> MAAQLSEQLAELEKRSGGRLGVAVLDTATGRRIAYRGDERFPMCSTFKALLAAAVLARVDQGKERLDRRITYGKEDLVDYSPVTEKHVGDGMTVAELCEAAITLSDNTAANLLLEALGGPAALTAFLRSIGDEVTRLDRWEPELNEAAPGDPRDTTTPAAMAATLRTLLLGDALSPASRQQLVDWLVANKTGDKRLRAGLPADWRVGDKTGTGGHGTTNDIAVIWPPGRAPIVVTVYLTESQVDA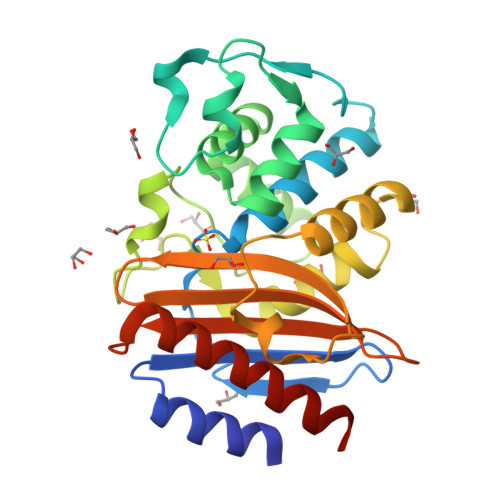DARDAVIAEVGRLVVEAFHHHHHH>[2x]MRSRRVDVMDVMNRLILAMDLMNRDDALRVTGEVREYIDTVKIGYPLVLSEGMDIIAEFRKRFGCRIIADFKVADIPETNEKICRATFKAGADAI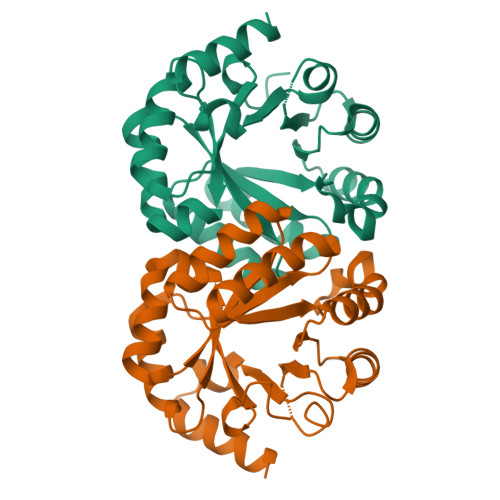IVHGFPGADSVRACLNVAEEMGREVFLLTEMSHPGAEMFIQGAADEIARMGVDLGVKNYVGPSTRPERLSRLREIIGQDSFLISPGAGAQGGDPGETLRFADAAIVGRSIYLADNPAAAAAGIIESIKDLLNP>[2x]MLLNALASLGHKGIKTLRTFGRAGLMLFNALVGKPEFRKHAPLLVRQLYNVGVLSMLIIVVSGVFIGMVLGLQGYLVLTTYSAETSLGMLVALSLLRELGPVVAALLFAGRAGSALTAEIGLMRATEQLSSMEMMAVDPLRRVISPRFWAGVISLPLLTVIFVAVGIWGGSLVGVSWKGIDSGFFWSAMQNAVDWRMDLVNCLIKSVVFAITVTWISLFNGYDAIPTSAGISRATTRTVVHSSLAVLGLDFVLTALMFGN;>MEQSVANLVDMRDVSFTRGNRCIF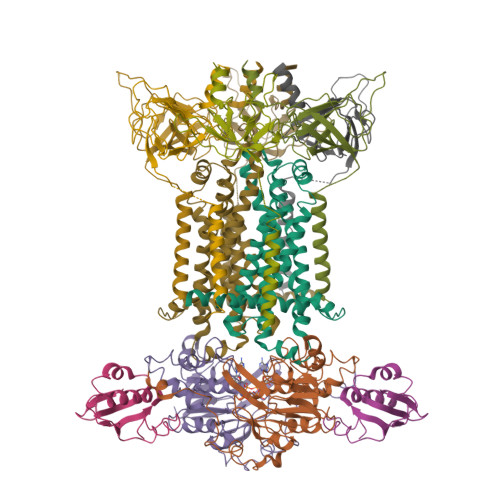DNISLTVPRGKITAIMGPSGIGKTTLLRLIGGQIAPDHGEILFDGENIPAMSRSRLYTVRKRMSMLFQSGALFTDMNVFDNVAYPLREHTQLPAPLLHSTVMMKLEAVGLRGAAKLMPSELSGGMARRAALARAIALEPDLIMFDQPFVGQDPITMGVLVKLISELNSALGVTCVVVSHDVPEVLSIADHAWILADKKIVAHGSAQALQANPDPRVRQFLDGIADGPVPFRYPAGDYHADLLPGS[2x];>MSESLSWMQTGDTLALSGELDQDVLLPLWEMREEAVKGITCIDLSRVSRVDTGGLALLLHLIDLAKKQGNNVTLQGVNDKVYTLAKLYNLPADVLPR[2x];>[6x]MQTKKNEIWVGIFLLAALLAALFVCLKAANVTSIRTEPTYTLYATFDNIGGLKARSPVSIGGVVVGRVADITLDPKTYLPRVTLEIEQRYNHIPDTSSLSIRTSGLLGEQYLALNVGFEDPELGTAILKDGDTIQDTKSAMVLEDLIGQFLYGSKGDDNKNSGDAPAAAPGNNETTEPVGTTK> AQT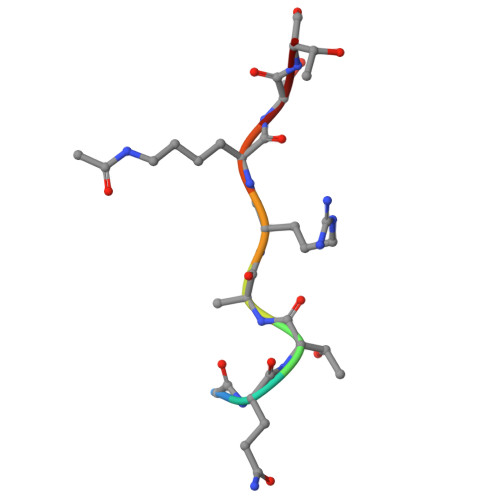ARKST> MTNPSPH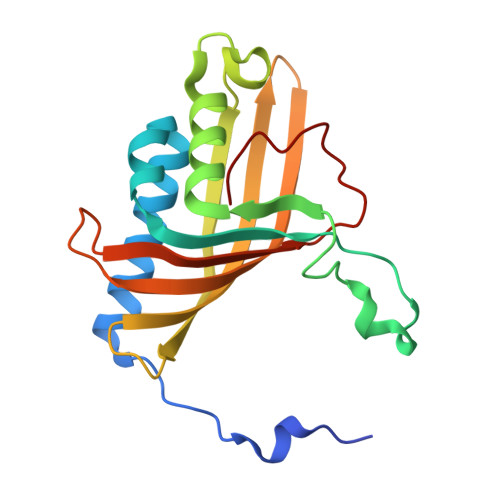FFKTFEWPSKAAGLELQNEIEQFYYREAQLLDHRAYEAWFALLDKDIHYFMPLRTNRMIREGELEYSGDQDLAHFDETHETMYGRIRKVTSDVGWAENPPSRTRHLVSNVIVKETATPDTFEVNSAFILYRNRLERQVDIFAGERRDVLRRADNNLGFSIAKRTILLDASTLLSNNLSMFF>RTAPSGSEYRHPGASDRPQPTAMNSIVMETGNTKNSALMAKKAPTMPKPQWHPPWKLYRVISGHLGWVRCIAVEPGNQWFVTGSADRTIKIWDLASGKLKLSLTGHISTVRGVIVSTRSPYLFSCGEDKQVKCWDLEYNKVIRHYHGHLSAVYGLDLHPTIDVLVTCSRDSTARIWDVRTKASVHTLSGHTNAVATVRCQAAEPQIITGSHDTTIRLWDLVAGKTRVTLTNHKKSVRAVVLHPRHYTFASGSPDNIKQWKFPDGSFIQNLSGHNAIINTLTVNSDGVLVSGADNGTMHLWDWRTGYNFQRVHAAVQPGSLDSESGIFACAFDQSESRLLTAEADKTIKVYREDDTATEETHPVSWKPEIIKRKRF[4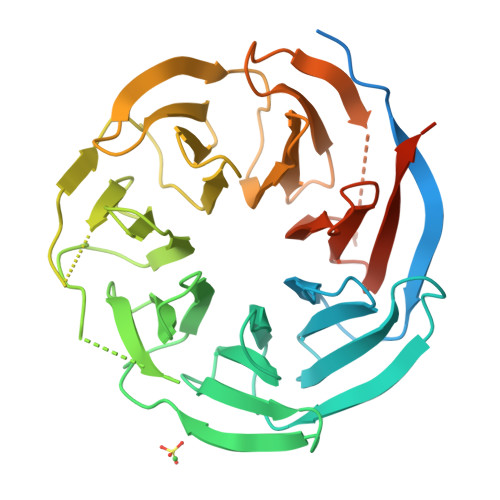x]>SDPAHTATAPGGLSAKAPAMTPLMLDTSSRKLVAWDGTTDGAAVGILAVAADQTSTTLTFYKSGTFRYEDVLWPEAASDET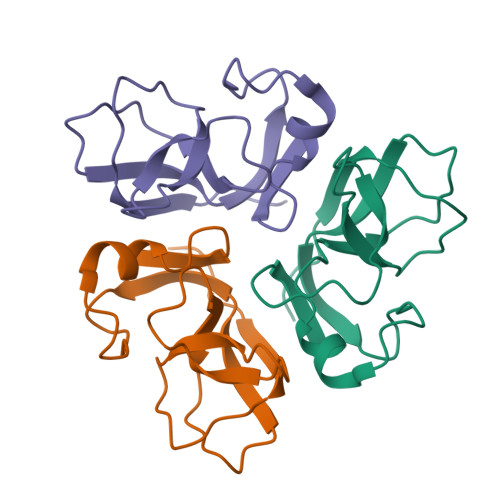KKRTAFAGTAISIV[6x]>AMDPEFMDAAIRQSLAKLGVQSTEIQASPVAGMKTVLTHSGVLYVTDDGKHIIQGPMYDVSGAHPVNVTNKLLMSQLNALEKEMIVYKAPDEKHVITVFTDITCGYCHKLHEEMKDYNALGITVRYLAFPAQGLESQAEQDMKSIWCAKDKNKAFDDAMAGKGVKPASCDVNIADHYALGVQLGVSGTPAIVLSNGYVVPGYQ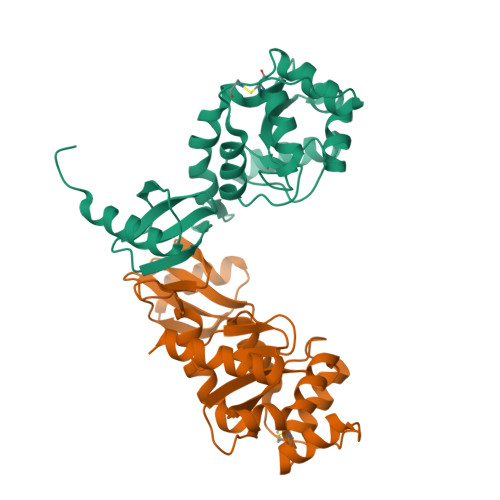GPKEMKAFLDEHQKQTSGK[2x]N-[(3M)-3-{6-[(3R)-3-methoxyoxolan-3-yl]pyridin-2-yl}-1-methyl-1H-pyrrolo[2,3-c]pyridin-5-yl]urea | C19 H21 N5 O3 | 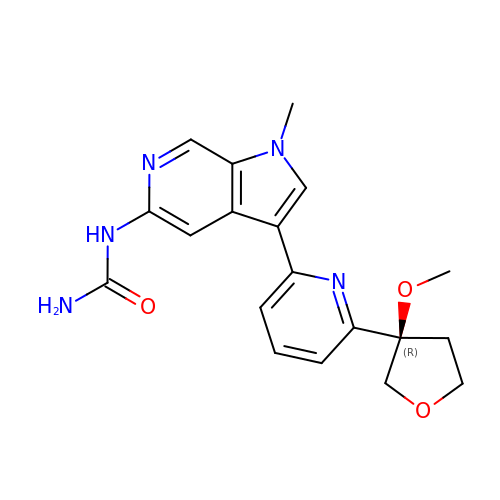LBFKCADAEOIHNK-IBGZPJMESA-N> M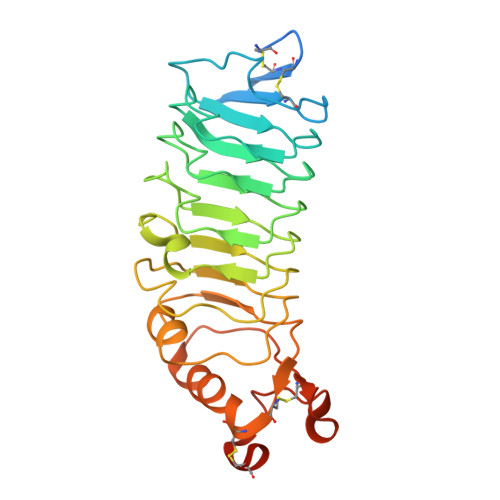LSGVWFLSVLTVAGILQTESRKTAKDICKIRCLCEEKENVLNINCENKGFTTVSLLQPPQYRIYQLFLNGNLLTRLYPNEFVNYSNAVTLHLGNNGLQEIRPGAFSGLKTLKRLHLNNNKLEVLREDTFLGLESLEYLQADYNYISTIEAGAFSKLNKLKVLILNDNLLLSLPSNVFRFVLLTHLDLRGNRLKVMPFAGVLEHIGGIMEIQLEENPWNCTCDLLPLKAWLDTITVFVGEIVCETPFRLHGKDVTQLTRQDLCPRKHHHHHH>LDRADILYNIRQTSRPDVIPTQRDRPVAVSVSLKFINILEVNEITNEVDVVFWQQTTWSDRTLAWNSSHSPDQVSVPISSLWVPDLAAYNAISKPEVLTPQLARVVSDGEVLYMPSIRQRFSCDVSGVDTESGATCRIKIGSWTHHSREISVDPTTENSDDSEYFSQYSRFEILDVTQKKNSVTYSCCPEAYEDVEVSLNFRKKGRSEIL[5x];>[5x]IRCFITPDITSKDCPNGHVCYTKTWCDAFCSIRGKRVDL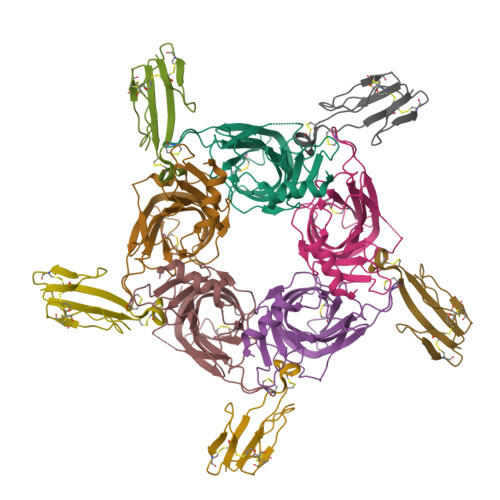GCAATCPTVKTGVDIQCCSTDNCNPFPTRKRP2-[(dibenzo[b,d]furan-2-yl)oxy]ethan-1-amine | C14 H13 N O2 | 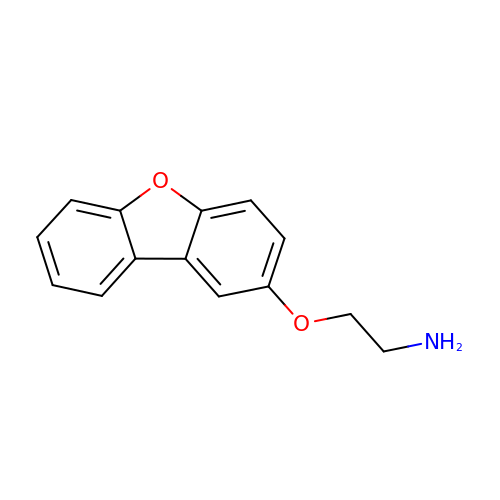LFVBNMSDBXKNRO-UHFFFAOYSA-N> MVKQIESKTAFQEALDAAGDKLVVVDFSATWCGPCKMIKPFFHSLSEKYSNVIFLEVDVDDCQDVASECEVKCM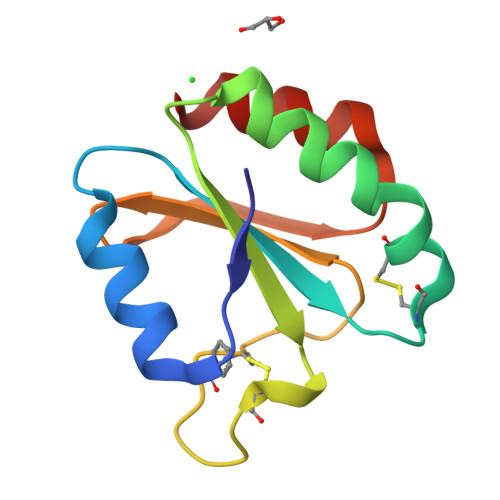PTFQFFKKGQKVGEFSGANKEKLEATINELV~{N}-cyclopropyl-2-methyl-5-phenyl-pyrazole-3-carboxamide | C14 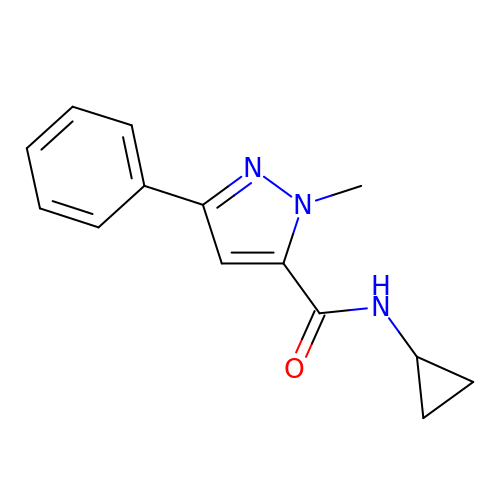H15 N3 O | YAWQTWUACTVACS-UHFFFAOYSA-N> GPLGSRPFKCSVCEKTYKDPATLRQHEKTHWLTRPFPCNI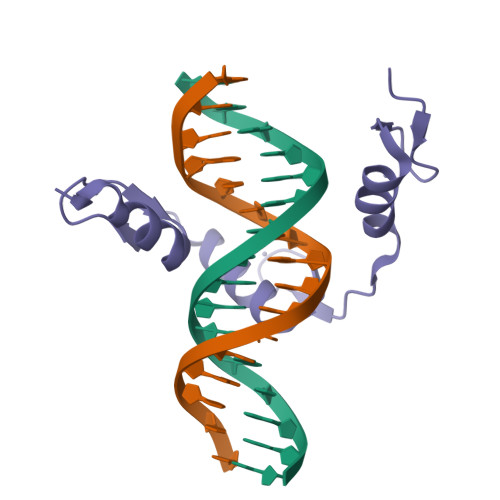CGKMFTQRGTMTRHMRSHLGLKPFACDECGMRFTRQYRLTEHMRVHSGEKPYECQLCGGKFTQQRNLISHLRMHTSPS> MAHHHHHHMSGIAAGRLAEERKAWRKNHPFGFIAKPSSNPDGTRNLFIWECAIPGKKGTIWEGGLYKIRMQFKDDYPSTPPKCKFDPPLFHPNVYPSGTVCLS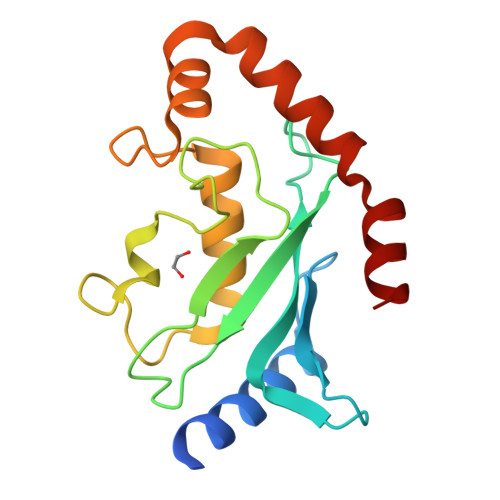ILDENKDWKPSISVRQLLIGIQDLLTNPNVDDPAQADAYQIYCQNRVEYEKRVRRQAQQFSAEIVQRQMLDN(2S)-2-azanyl-6-(phenylmethoxycarbonylamino)hexanoic acid | C14 H20 N2 O4 | 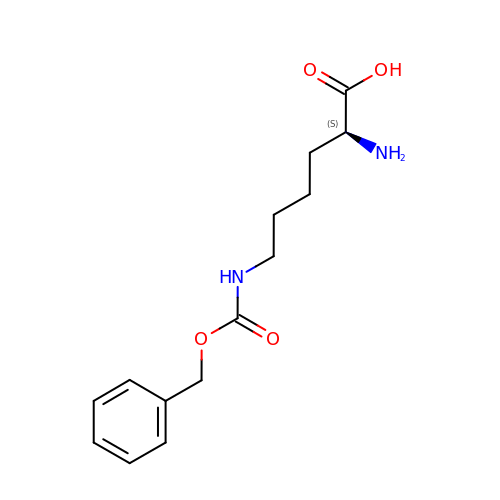CKGCFBNYQJDIGS-LBPRGKRZSA-N> GQGVYTYEDGGVLQGTYVDGELNGPAQEYDTDGRLIFKGQYKDNIRHGVCWIYYPDGGSLVGEVNEDGEMTGEKIAYVYPDERTALYGKFIDGEMIEGKLATLMSTEEGRPHFELMPGNSVYHFDKSTSSCISTNALLPDPYESERVYVAESLISSAGEGLFSKVAVGPNTVMSFYNGVRITHQE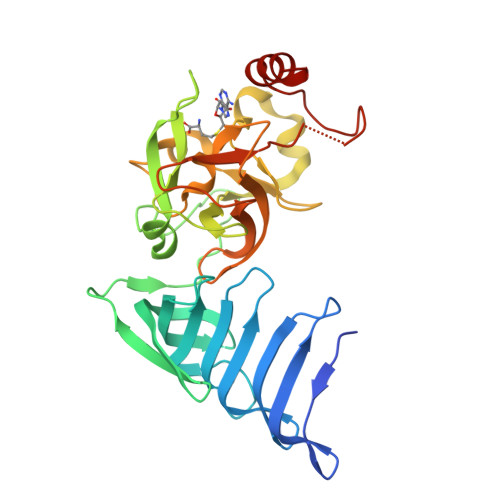VDSRDWALNGNTLSLDEETVIDVPEPYNHVSKYCASLGHKANHSFTPNCIYDMFVHPRFGPIKCIRTLRAVEADEELTVAYGYDHSPPGKSGPEAPEWYQVELKAFQATQQK DesF-3R/4076 | C26 H30 N6 O4 | 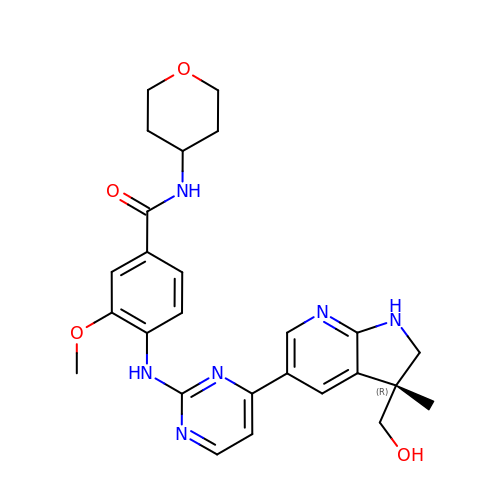SSABYHFPMHHFLH-AREMUKBSSA-N>MAKPLTDQEKRRQISIRGIVGVENVAELKKSFNRHLHFTLVKDRNVATTRDYYFALAHTVRDHLVGRWIRTQQHYYDKCPKRVYYLSLEFYMGRTLQNTMINLGLQNACDEAIYQLGLDIEELEEIEEDAGLGNGGLGRLAACFLDSMATLGLAAYGYGIRYEYGIFNQKIRDGWQVEEADDWLRYGNPWEKSRPEFMLPVHFYGKVEHTNTGTKWIDTQVVLALPYDTPVPGYMNNTVNTMRLWSARAPNDFNLRDFNVGDYIQAVLDRNLAENISRVLYPNDNFFEGKELRLKQEYFVVAATLQDIIRRFKASKFGSTRGAGTVFDAFPDQVAIQLNDTHPALAIPELMRIFVDIEKLPWSKAWELTQKTFAYTNHTVLPEALERWPVDLVEKLLPRHLEIIYEINQKHLDRIVALFPKDVDRLRRMSLIEEEGSKRINMAHLCIVGSHAVNGVAKIHSDIVKTKVFKDFSELEPDKFQNKTNGITPRRWLLLCNPGLAELIAEKIGEDYVKDLSQLTKLHSFLGDDVFLRELAKVKQENKLKFSQFLETEYKVKINPSSMFDVQVK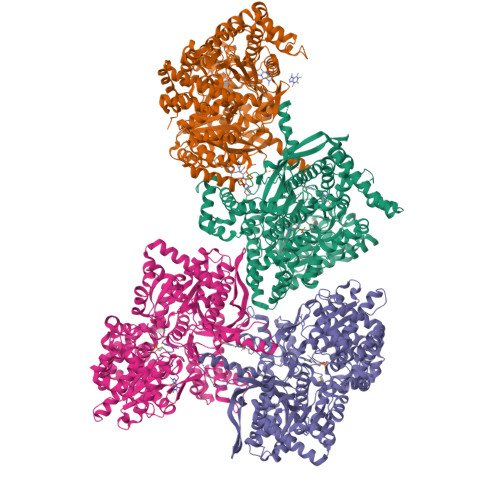RIHEYKRQLLNCLHVITMYNRIKKDPKKLFVPRTVIIGGKAAPGYHMAKMIIKLITSVADVVNNDPMVGSKLKVIFLENYRVSLAEKVIPATDLSEQISTAGTEASGTGNMKFMLNGALTIGTMDGANVEMAEEAGEENLFIFGMRIDDVAALDKKGYEAKEYYEALPELKLVIDQIDNGFFSPKQPDLFKDIINMLFYHDRFKVFADYEAYVKCQDKVSQLYMNPKAWNTMVLKNIAASGKFSSDRTIKEYAQNIWNVEPSDLKISLSNESNKVNGN[2x]> KPSSVAFWYAEQPPLAELSQFDWVVLEPGHADAADIAYLKAQGSTPFAYLSVGEFDGDTAELAGAGLEEGASAVRNDAWHSQVMDLSSSVWREHLFSRAAELRRQGYAGLFLDTLDSFQLQSEDRHEPQRQALVSLLAELHRREPQLSLFFNRGFEVLPELPGVASAVAVESIHAGWEAASSRYRTVSQEDRDWLQPHLEALRAQGVPLVAIEYLPPERREEARELAA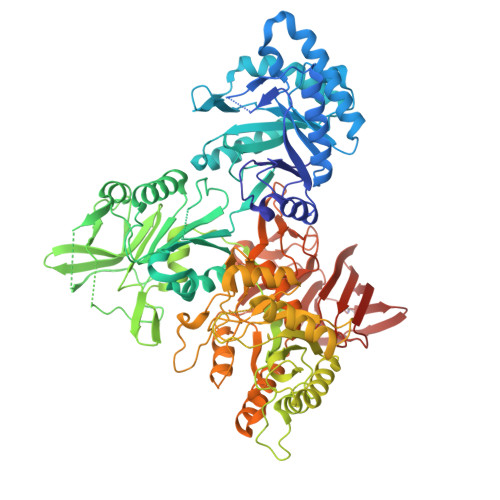RLVKEGFIPYVTTPALDTLGVGSLEVQPRRIALVYDPREGELESNPGHVMLGGLLEYLGYRVDYWPAGEALPQRPLKGLYAGVVIWMTSGPPSASDSFHAWLNARIDEQVPIAFLAGLPVDNDGLLQRLGMRRLSQPLRGEPRLEFHDQSLLGAFEAPLRLRTRDLPALTVTDPQLTQAALVLEHGGRRYVPVATGTWGGIALAPYLVEEALDHRRWIIDPFAFIQRAFALPPLPSPDVTTENGRRVATVHIDGDGFVSRAEVPGTPYAGQQVLEAFIRPYPLLTSVSVVEGEVGPKGMYPHLSKELEPIARRIFADPKVEVASHTFSHPFFWQPEKAAQSDDFDPQYGLMMKIPGYEVLDMRREVVGTRDYINQRLTTPEKPVKMIFWSGDALPDAETIKLAYDSGLPNVNGGNTMLTKAYPSLTGLYPLIRPTSGGVQYYAPIINENVYTNLWTGPYYGFRDVLDTFALTDQPRRLRGLHLYYHFYSGTKQASIRAMHQIYAEMLRQQPLSLWMSDYVRRLEGLHCASLARRADGRWQLRGLAGLRTLRLDPALGWPDLARSKGVAGVRDLPQGRYVHLSRADALLALRSSRDPRPALEEANLPLTAWEYRSASQVSFSFAGELPLQFSVRAAGPCRVTVAGQSFQGKEHDGLWRFQLPMKQVRDGQLVC Consequently, trypanosomatids possess multiple biopterin and folate transporters with salvage pathways to convert them into the reduced cofactors 5,6,7,8-tetrahydrobiopterin (H4B) and 5,6,7,8-tetrahydrofolate (H4F) by means of pteridine reductase 1 (PTR1, EC 1.5.1.33) and the bifunctional, nicotinamide adenine dinucleotide phosphate (NADPH)-dependent enzyme dihydrofolate reductase–thymidylate synthase (DHFR-TS, ECs 1.5.1.4 and 2.1.1.45, respectively). [10,11], PTR1, a broad-specificity, short-chain dehydrogenase, can reduce dihydrofolate (H2F) to H4F, thereby circumventing inhibition of DHFR-TS. Whereas DHFR-TS enzymes are restricted in their substrate repertoire, primarily reducing H2F to H4F, PTR1 can reduce numerous pterins and folates.

The ultimate validation of this novel screening assay was confirmed on demonstration that compounds identified as actives using the new assay were in fact legitimately binding to TbPTR1. We have shown, using cocrystallization studies, that an example small molecule identified using the screening assay described here binds to TbPTR1 through interactions within the pterin binding pocket in a manner similar to that observed for MTX. The binding mode of the ligand is similar to that observed for MTX bound to TbPTR1, with the diaminoquinazoline ring of DDD00066641 sandwiched between the nicotinamide ring of the cofactor and the side chain of Phe97. The diaminoquinazoline ring of DDD00066641 also shows an identical pattern of H-bond interactions to the protein chain and cofactor, as observed for the pteridine ring of MTX. The ligand forms three H-bonds to the protein: the 2 amino group interacting with both the main chain carbonyl and side chain hydroxyl of Ser95 and the 4 amino group interacting with the side chain hydroxyl of Tyr174. Two H-bonds are also formed via the N1 atom to the α-phosphate group and from the N3 atom to the nicotinamide ribose 2′ hydroxyl. The hydrophobic toluene substituent packs against a hydrophobic surface formed by the side chains of Leu209, Pro210, Met213, and Tyr221. Routine cocrystallization studies with TbPTR1 across these series have repeatedly confirmed the binding mode revealed for DDD00066641. Furthermore, the structure–activity relationships developed and informed by data generated by the screening assay conform well to the binding modes identified for multiple series through similar cocrystallization studies.

>[4x]MEAPAAVVTGAAKRIGRAIAVKLHQTGYRVVIHYHNSAEAAVSLADELNKERSNTAVVCQADLTNSNVLPASCEEIINSCFRAFGRCDVLVNNASAFYPTPLVQGDHEDNSNGKTVETQVAELIGTNAIAPFLLTMSFAQRQKGTNPNCTSSNLSIVNLCDAMVDQPCMAFSLYNMGKHALVGLTQSAALELAPYGIRVNGVAPGVSLLPVAMGEEEKDKWRRKVPLGRREASAEQIADAVIFLVSGSAQYITGSIIKVDGGLSLVHA>PAARVEYIAPWWVVWLHSVPHLGLRLQRVDSTFSPGDETYQESLLFLGVLAAIGLGLNLI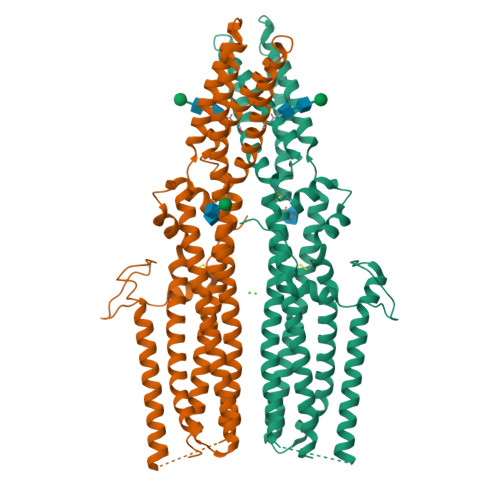FLTVYLVCTCCCRRDHTVQTKQQESCCVTWTAVVAGLLCCAAVGVGFYGNSETNDGMHQLIYSLDNANHTFSGMDELVSANTQRMKVDLEQHLARLSEIIAARGDYIQTLKFMQQMAGNVVSQLSGLPVWREVTTQLTKLSHQTAYVEYYRWLSYLLLFILDLVICLVTCLGLARRSKCLLASMLCCGILTLILSWASLAADAAAAVGTSDFCMAPDIYILNNTGSQINSEVTRYYLHCSQSLISPFQQSLTTFQRSLTTMQIQVGGLLQFAVPLFPTAEKDLLGIQLLLNNSEISLHQLTAMLDCRGLHKDYLDALTGICYDGIEGLLFLGLFSLLAALAFSTLTCAGPRAWKYFINRDRDYDDIDDDDPFNPQARRIAAHNPTRGQLHSFCSYSSGLGSQCSLQPPSQTISNAPVSEYMNQAILFGGNPRYENVPLIGRGSPPPTYSPSMRPTYMSVADEHLRHYEFPSSNSLEVLFQ[2x]>MAKFFIDRPIFAWVISIFIIAAGIFGIKSLPVSQYPSVAAPTITLHAIYPGASAQVMEGSVLSVIERNMNGVEGLDYMSTSADSSGSGSVSLTFTPDTDENLAQVEVQNKLSEVLSTLPATVQQYGVTVSKARSNFLMIVMLSSDVQSTEEMNDYAQRNVVPELQRIEGVGQVRLFGAQRAMRIWVDPKKLQNYNLSFADVGSALSAQNIQISAGSIGSLPAVRGQTVTATVTAQGQLGTAEEFGNVILRANTDGSNIYLKDVAKVGLGMEDYSSSTRLNGVNTTGMAVMLSNSGNAMATAKAVKERLAVLEKYFPQGMSWKTPYDTSKFVEISIEKVIHTLIEAMVLVFVVMYLFLQNIRYTLIPTIVVPISLLGGFAFISYMGMSINVLTMFAMILVIGIVVDDAIVVVENVERIMAGEGLPPKEATKKAMGQISGAVIGITAVLISVFVPLAMFSGAAGNIYKQFALTMASSIAFSAFLALTLTPALCATMLKTIPKGHHEEKKGFFGWFNKKFDSWTHGYEGRVAKVLRKTFRMMVVYIGLAVVGVFLFMRLPTSFLPTEDQGFVMVSVQLPAGATKERTDATLAQVTQLAKSIPEIENIITVSGFSFSGSGQNMAMGFAILKDWNERTASGSDAVAVAGKLTGMMMGTLKDGFGIAVVPPPILELGNGSGLSINLQDRNNTGHTALLAKRNELIQKMRASGLFDPSTVRAGGLEDSPQLKIDINRAAAAAQGVSFADIRTALASALSSSYVSDFPNQGRLQRVMVQADGDARMQPADILNLTVPNSSGIAVPLSSIATVSWQMGTEQSVRFNGYPAMELSGSPATGVSTGQAMEAVQKMVDELGSGYSLEWGGQSREEAKGGSQTIALYALAAVAVFLVLAALYESWSIPLAVLLVMPLGLAGAAAGVTGRNLFEGLLGSVPSFANDIYFQVGFVTVMGLSAKNAILIIEFAKDLQAQGKSAVEAALEAARLRFRPIIMTSFAFILGVVPLYIAGGASSASQRAIGTTVFWGMLIGTLLSVFLVPLFYVVVRKFFKETAHEHEMAVRHASKAGITGSDDKQY[3x];> CTNEDGKPC

In Neisseria gonorrhoeae, the best-characterized and most clinically important multidrug efflux system is the multiple transferrable resistance (MtrCDE) tripartite efflux pump, a member of the widely distributed resistance-nodulation-cell division (RND) superfamily in Gram-negative bacteria. N. gonorrhoeae MtrD contains multidrug binding sites and a proton relay network that generates the proton motive force (PMF) essential for drug expulsion from the bacterial cell. This multidrug efflux pump couples with the MtrC periplasmic membrane fusion protein and the MtrE outer membrane channel to actively extrude antimicrobials and mediate drug resistance. Based on the cryo-EM structures of MtrDCR103-CASP, MtrDCR103-Col, and MtrDCR103-LL, we observed that MtrDCR103 employs different binding modes to anchor linear and cyclic peptides.

To further enhance the stability of ADP6, we covalently cyclized this peptide by cross-linking its N- and C-terminal cysteines to form CASP. We then incubated 2 μM the MtrDCR103-nanodisc sample with 100 μM CASP for 2 h to form the MtrDCR103-CASP complex and determined the MtrDCR103-CASP structure using single-particle cryo-EM. The reconstituted sample led to a cryo-EM map at a nominal resolution of 2.95 Å, allowing us to obtain a structural model of this pump-peptide complex. In MtrDCR103-CASP, the three MtrDCR103 protomers display the typical “access,” “binding,” and “extrusion” conformations. An extra density corresponding to the CASP molecule is observed to anchor at the distal drug binding pocket of the binding protomer. No extra densities are found in the access and extrusion protomers. It appears that a number of residues are engaged in anchoring this peptide, including those within the entrance drug binding site, F-loop, proximal drug binding site, G-loop, distal drug binding site, and hydrophobic patch. Within 4.5 Å of bound CASP, there are 19 residues participating in binding. These residues are H46, F136, I139, M141, R174, F176, S275, T277, A288, M290, Y325, F568, I605, V607, F610, F612, F623, I625, and L668. Particularly, we found that the side chains of R174 and T277 are involved in forming two hydrogen bonds with bound CASP to further secure peptide binding.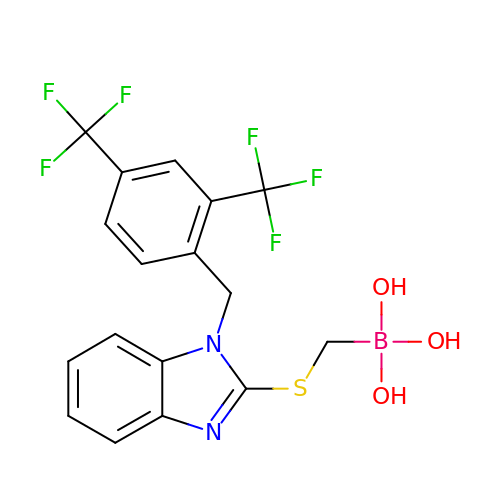[1-[[2,4-bis(trifluoromethyl)phenyl]methyl]benzimidazol-2-yl]sulfanylmethyl-$l^{3}-oxidanyl-bis(oxidanyl)boron | C17 H14 B F6 N2 O3 S | KHOQXIARLAATHE-UHFFFAOYSA-N> GEFSGPPVERCGVLSKWTNYIHGWQDRWVVLKNNALSYYKSEDETEYGCRGSICLSKAVITPHDFDECRFDISVNDSVWYLRAQDPDHRQQWIDAIEQHKTESGYG;> GHMAMEFSSVGTHRFVQKVEEMVQNHMTYSLQDVGGDANWQLVVEEGEMKVYRREVEENGIVLDPLKATHAVKGVTGHEVCNYFWNVDVRNDWETTIENFHVVETLADNAIIIYQTH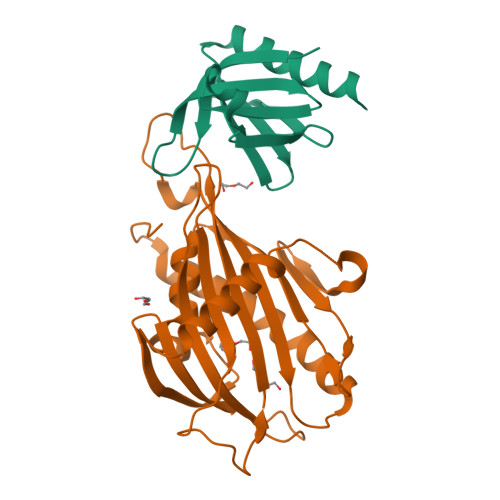KRVWPASQRDVLYLSVIRKIPALTENDPETWIVCNFSVDHDSAPLNNRCVRAKINVAMICQTLVSPPEGNQEISRDNILCKITYVANVNPGGWAPASVLRAVAKREYPKFLKRFTSYVQEKTAGKPILF>GSSHHHHHHSSGLVPRGSHMASTEAAAQPHALPADAPDIAPERDLLSKFDGLIAERQKLLDSGVTDPFAIVMEQVKSPTEAVIRGKDTILLGTYNYMGMTFDPDVIAAGKEALEKFGSGTNGSRMLNGTFHDHMEVEQALRDFYGTTGAIVFSTGYMANLGIISTLAGKGEYVILDADSHASIYDGCQQGNAEIVRFRHNSVEDLDKRLGRLPKEPAKLVVLEGVYSMLGDIAPLKEMVAVAKKHGAMVLVDEAHSMGFFGPNGRGVYEAQGLEGQIDFVVGTFSASVGTVGGFVVSNHPKFEAVRLACRPYIFTASLPPSVVATATTSIRKLMTAHEKRERLWSNARALHGGLKAMGFRLGTETCDSAIVAVMLEDQEQAAMMWQALLDGGLYVNMARPPATPAGTFLLRCSICAEHTPAQIQTV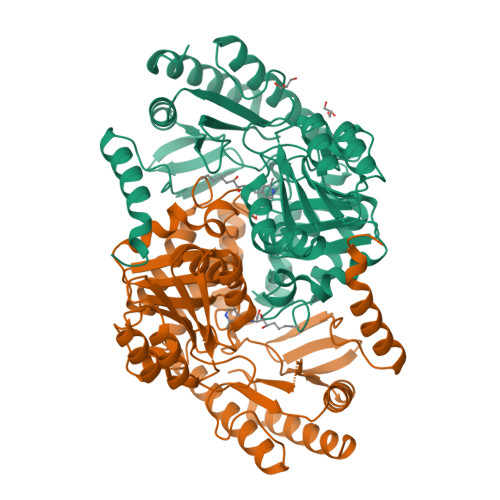LGMFQAAGRAVGVIGL[2x]> MGSDRSCVLSVFQTILKLVIFVAIFGAAISSRLFAVIKFESIIHEFDPWFNYRATKYLVNNSFYKFLNWFDDRTWYPLGRVTGGTLYPGLMTTSAFIWHALRNWLGLPIDIRNVCVLFAPLFSGVTAWATYEFTKEIKDASAGLLAAGFIAIVPGYISRSVAGSYDNEAIAITLLMVTFMFWIKAQKTGSIMHATCAALFYFYMVSAWGGYVFITNLIPLHVFLLILMGRYSSKLYSAYTTWYAIGTVASMQIPFVGFLPIRSNDHMAALGVFGLIQIVAFGDFVKGQISTAKFKVIMMVSLFLILVLGVVGLSALTYMGLIAPWTGRFYSLWDTNYAKIHIPIIASVSEHQPVSWPAFFFDTHFLIWLFPAGVFLLFLDLKDEHVFVIAYSVLCSYFAGVMVRLMLTLTPVICVSAAVALSKIFDIYLDFKTSDRKYAIKPAALLAKLIVSGSFIFYLYLFVFHSTWVTRTAYSSPSVVLPSQTPDGKLALIDDFREAYYWLRMNSDEDSKVAAWWDYGYQIGGMADRTTLVDNNTWNNTHIAIVGKAMASPEEKSYEILKEHDVDYVLVIFGGLIGFGGDDINKFLWMIRISEGIWPEEIKERDFYTAEGEYRVDARASETMRNSLLYKMSYKDFPQLFNGGQATDRVRQQMITPLDVPPLDYFDEVFTSENWMVRIYQLKKDDAQGRTLRDVGELTRSSTKTRRSIKRPELGLRV;> MISDEQLNSLAITFGIVMMTLIVIYHAVDSTMSPKNRTLQVDGGSGGSLEVLFQGPTETSQVAPA;> MTYEQLYKEFHSSKSFQPFIHLDTQPKFAICGLIVTLAVLSSALFAVGSKSSYIKKLFFYTILSVIGSLFAGLTTVFASNSFGVYV;> MAKAPKANTPKVTSTSSAVLTDFQETFKTSKRAYFAQIEKYPKLKLIDTFCFFLVLLGVIQCTFIILIRDNFPFNAFLAGFIICVGQFVLLMSLRLQLCNSFPGISKNRAFAEFIVASLILHFVCLHFIN;> MRQVWFSWIVGLFLCFFNVSSAAQYEPPATWENVDYKRTIDVSNAYISETIEITIKNIASEPATEYFTAFESGIFSKVSFFSAYFTNEATFLNSQLLANSTTAPGDDGESEIRYGIIQFPNAISPQEEVSLVIKSFYNTVGIPYPEHVGMSEEQHLLWETNRLPLSAYDTKKASFTLIGSSSFEEYHPPNDESLLGKANGNSFEFGPWEDIPRFSSNETLAIVYSHNAPLNQVVNLRRDIWLSHWASTIQFEEYYELTNKAAKLSKGFSRLELMKQIQTQNMRQTHFVTVLDMLLPEGATDHYFTDLVGLVSTSHAERDHFFIRPRFPIFGGWNYNFTVGWTNKLSDFLHVSSGSDEKFVASIPILNGPPDTVYDNVELSVFLPEGAEIFDIDSPVPFTNVSIETQKSYFDLNKGHVKLTFSYRNLISQVANGQVLIKYDYPKSSFFKKPLSIACYIFTALMGVFVLKTLNMNVTN;> MQFFKTLAALVSCISFVLAYVAQDVHVSFPSTAGKSRVMIGKVEPRIGIDETVPTTITVEDPNEVIQVNFAIESTNKPFQNTLLIGLPNKNLEMAFEPEIKDNGKLSMYKYRIDLAKLDAALLQEASRSPEPIKATLILASSTAKPKENLFREILQLNLNFDVDHSDSSLVDKFGIKPEIHHIFHAEPKRVAKPIAVIFVLIIFITILSLIVTWLNSCAAAFNNIPTGVTAVYFLGFIATIVGFEVIFARYYLGTSIFETLFSSLYLGAPGLLTSTKFLRSFG;> MRTDWNFFFCILLQAIFVVGTQTSRTLVLYDQSTEPLEEYSVYLKDLEQRNYKLEYLDINSTSTTVDLYDKEQRLFDNIIVFPTKGGKNLARQIPVKQLIKFFENEGNILCMSSPGAVPNTIRLFLNELGIYPSPKGHVIRDYFSPSSEELVVSSNHLLNKYVYNARKSEDFVFGESSAALLENREQIVPILNAPRTSFTESKGKCNSWTSGSQGFLVVGFQNLNNARLVWIGSSDFLKNKNQDSNQEFAKELLKWTFNEKSVIKSVHAVHSHADGTSYDEEPYKIKDKVIYSVGFSEWNGEEWL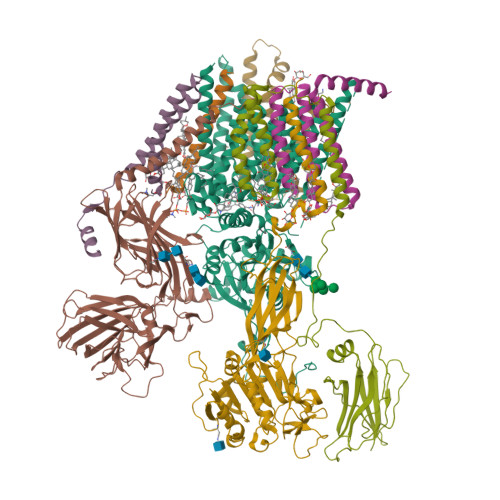PHIADDIQFELRQVDPYYRLTLSPSGNDSETQYYTTGEFILPDRHGVFTFLTDYRKIGLSFTTDKDVKAIRHLANDEYPRSWEISNSWVYISAICGVIVAWIFFVVSFVTTSSVGKKLETFKKTN;> MNWLFLVSLVFFCGVSTHPALAMSSNRLLKLANKSPKKIIPLKDSSFENILAPPHENAYIVALFTATAPEIGCSLCLELESEYDTIVASWFDDHPDAKSSNSDTSIFFTKVNLEDPSKTIPKAFQFFQLNNVPRLFIFKPNSPSILDHSVISISTDTGSERMKQIIQAIKQFSQVNDFSLHLPMDWTPIITSTIITFITVLLFKKQSKLMFSIISSRIIWATLSTFFIICMISAYMFNQIRNTQLAGVGPKGEVMYFLPNEFQHQFAIETQVMVLIYGTLAALVVVLVKGIQFLRSHLYPETKKAYFIDAILASFCALFIYVFFAALTTVFTIKSPAYPFPLLRLSAPFK;> YANATSA T3SS2 expression is regulated by VtrA–VtrC, a member of a newly described superfamily of bacterial “co-component” signaling systems. The transcription factor component (VtrA) includes an N-terminal helix–turn–helix DNA-binding domain (DBD), a single transmembrane helix, and a C-terminal periplasmic domain, whereas the sensor component (VtrC) includes a transmembrane helix followed by a lipocalin-like periplasmic domain. In the case of VtrA–VtrC, VtrA functions as a membrane-bound transcription factor, whereas VtrC in complex with VtrA senses bile. When VtrA–VtrC bind bile acids in the periplasm, the VtrA DBD is activated in the cytoplasm.

We purified the VtrA–VtrC periplasmic domain complex in the presence of CDC, crystallized this complex in space group C2, and obtained the X-ray structure. We then solved the structure of the VtrA–VtrC complex bound with CDC and observed that CDC binds in the same hydrophobic pocket of the VtrA–VtrC complex as TDC. Despite their common steroid nucleus, CDC is modified with an R1-OH that is absent in TDC. This unique CDC hydroxyl group forms a hydrogen bond with a water molecule that is also coordinated by VtrC H50 ND1 and Y151-OH. The backbone amide of VtrC Y151 forms a hydrogen bond with the 3α-OH of CDC, and VtrC Y81 makes van der Waals contacts with CDC. Specifically, the coordinated water molecule between H50, Y151, and the R2-OH of CDC increases the distance between the H50 and Y151 side chains, as compared with the TDC-bound structure, where they form a hydrogen bond. The key Fα S123 side chain makes a hydrogen bond with the R1-OH of TDC, which is lacking in CDC. Finally, the Y81-OH group shifts between 0.8 and 2.3 Å in the CDC-bound structure so that the aromatic side chain forms van der Waals contacts with both the five-membered ring and the carbon side chain from CDC. The position of the Fα helix containing residue S123 is impacted by crystal packing and shifts away from the CDC binding site in one heterodimer compared with the others in the asymmetric unit. Meanwhile, the lack of a hydrogen bond between CDC and S123 allows mobility in the Fα helix and alternates conformations dictated by the crystal contacts.

>[4x]MTAKDDYPSLSFQQDYVYIFSSDFQLSEELGVALINALSAKEIVPERLYVMLNDKTISFSFISKNKKSKNRVLSTEKKLNYKHISEYIVNEIEY;>MGSSHHHHHHSQDPVHFYETSYKYQAADSTYMHDVAINVSIKGNHFTSDIIIRELVKSENKNYYNVIGHGDIIQKNTHQYYLNFDNIDVYTGTNKANMKPYKEPTSISSLINKSNNIRVVYLSEEYVVVEFFFYDGQIITLHRY[4x]>MQPMTARFDLFVVGSGFFGLTIAERVATQLDKRVLVLERRPHIGGNAYSEAEPQTGIEVHKYGAHLFHTSNKRVWDYVRQFTDFTDYRHRVFAMHNGQAYQFPMGLGLVSQFFGKYFTPEQARQLIAEQAAEIDTADAQNLEEKAISLIGRPLYEAFVKGYTAKQWQTDPKELPAANITRLPVRYTFDNRYFSDTYEGLPTDGYTAWLQNMAADHRIEVRLNTDWFDVRGQLRPGSPAAPVVYTGPLDRYFDYAEGRLGWRTLDFEVEVLPIGDFQGTAVMNYNDLDVPYTRIHEF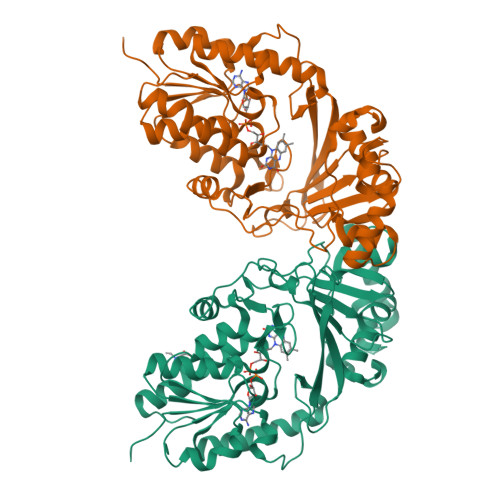RHFHPERDYPTDKTVIMREYSRFAEDDDEPYYPINTEADRALLATYRARAKSETASSKVLFGGRLGTYQYLDMHMAIASALNMYDNVLAPHLRDGVPLLQDGA[4x]> MHHHHHHSPLRVALYGFGNQNKEMAKMLVERKDVEIVAVISNKSNVGKDFGEVIGLAPQGILVTAGLDAAETLRTTNPQIAMLSTLSTVGDIESQLRACAENKVNVYTIAEELTFSWTSAPEKTKEMDELFKEHNVSLIGGGFLDGACCDMARTMAAMMHKIDKLDGGLQYNVDHYGQVLAIAHGVGLSEEEFYAENGPGWTSPTSYPKSYVYNMNDWFASAFGLTVIKTEEVKTPTKAPIELYSEAIGRAIPVGQCTGMIVTATTTTEEGVIIVEKQVGKCYEDGDEDMVFMNLEGNPTGGVGFTMKNPPTPAMTNTIAISRMFQTVDAPAGYITTDKLPTMEAYVHGRL

Native amine dehydrogenases (nat‐AmDHs) have recently emerged as a potentially valuable new reservoir of enzymes for the sustainable and selective synthesis of chiral amines, catalyzing the NAD(P)H‐dependent ammoniation of carbonyl compounds with high activity and selectivity. MATOUAmDH2, recently identified from the Marine Atlas of Tara Oceans Unigenes (MATOUv1) database of eukaryotic genes, displays exceptional catalytic performance against its best identified substrate, isobutyraldehyde, as well as having broader substrate scope than other nat‐AmDHs. In the interests of providing a platform for the rational engineering of this and other nat‐AmDHs, we have determined the structure of MATOUAmDH2 in complex with NADP+ and also with the cofactor and cyclohexylamine. The two‐domain structure of the MATOU monomer is similar to that observed with CfusAmDH and MsmeAmDH, with a largely N‐terminal Rossman fold domain (residues 8–158; 309–351) and a largely C‐terminal domain 159–309 comprising a seven‐stranded beta sheet.

Following subcloning and expression using pETYSBLIC‐3 C, which equips MATOUAmDH2 with a 12 amino acid extension leading to the hexahistidine tag at the N‐terminus, further crystals, formed in the presence of both NADP+ and the reaction product cyclohexylamine, were obtained, with an improved resolution of 2.08 Å. In this case the crystals were obtained in space group P321 with one molecule in the asymmetric unit, which was in the closed conformation equivalent to that observed with the C monomer of the NADP+‐only complex (rmsd of 0.40 Å over 340 Cα atoms). In this structure, the omit maps revealed clear electron density adjacent to E111, which was modelled and refined successfully as cyclohexylamine. The ligand was, as expected, positioned with its ring plane sandwiched between the nicotinamide ring of NADP+ and the side chain of Y171 and with its nitrogen atom 2.5 Ångstroms from the OE2 carboxylate atom of E111. The ligand cyclohexylamine (CHA) is also bound in a different orientation, with the cyclohexyl ring more in plane with the side chain of Y171 and the nicotinamide ring of NADP+. The resulting data were refined to a resolution of 2.08 Å and the experimental maps clearly showed density corresponding to CHA in the active site. The structure of MATOUAmDH2 in complex with cyclohexylamine suggests that the improved activity for the production of N‐methyl cyclohexylamine may be due to the increased space afforded by the L−A mutation in the roof of the active site, permitting improved binding of the relevant alkyl imine intermediate from solution for reduction. The acquisition of the MATOUAmDH2 structure in complex with cyclohexylamine permitted us to model substrates into the active site in order to rationalize the observed stereoselectivity of the enzyme. In doing so, we have used Autodock Vina to model the intermediate iminium 16 into the newly described active site of MATOUAmDH2 (SI Section 9).(2S)-2-(3,3-dimethylbutanoylamino)-N-[(2S)-1-[[(2S,3S)-3-hydroxy-4-[(4-iodophenyl)methylamino]-4-oxo-butan-2-yl]amino]-1,4-dioxo-4-pyrrol-1-yl-butan-2-yl]-3,3-dimethyl-butanamide 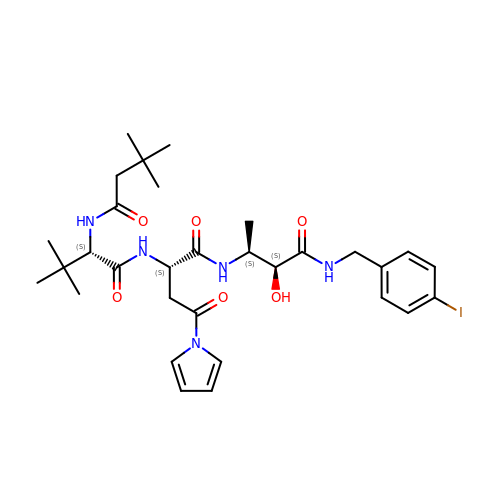| C31 H44 I N5 O6 | DUBMDYQWHSIBPD-FBESYSLLSA-N>[2x]MSEENVVYIGNKPVMNYVLAVVTQM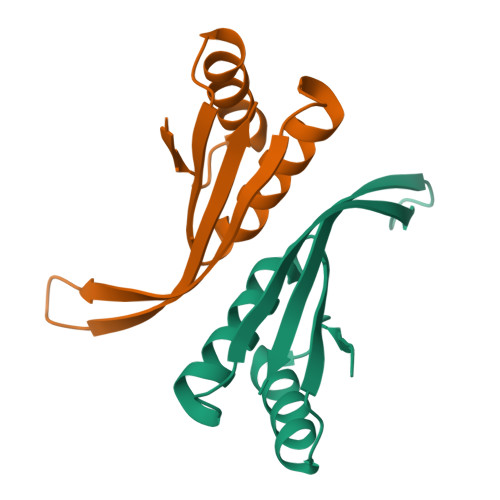NGGTSEVILKARGIAISRAVDVAEIVRNRFIPDIQIENIDICTEEIIGNEGTATNVSAIEIQLRKD> PPPPPPP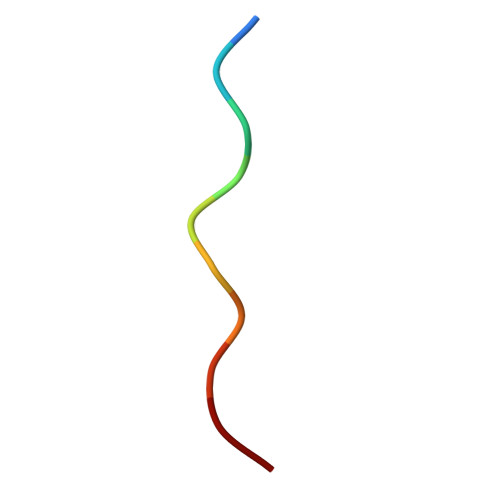PPL>MPLEPHFMPDFLGHAENPLREEEWARLNETVIQVARRSLVGRRILDIYGPLGAGVQTVPYDEFQGVSPGAVDIVGEQETAMVFTDARKFKTIPIIYKDFLLHWRDIEAARTHNMPLDVSAAAGAAALCAQQEDELIFYGDAR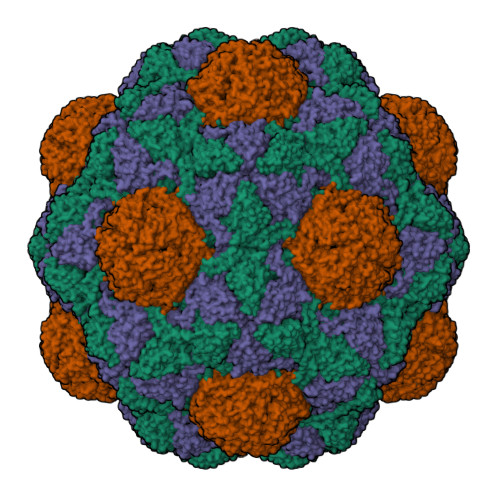LGYEGLMTANGRLTVPLGDWTSPGGGFQAIVEATRKLNEQGHFGPYAVVLSPRLYSQLHRIYEKTGVLEIETIRQLASDGVYQSNRLRGESGVVVSTGRENMDLAVSMDMVAAYLGASRMNHPFRVLEALLLRIKHPDAICTLEGAGATERR[3x];>PEKRLTVGSLRR[3x]>[2x]GSHMSRVQLALRVPDLEASIG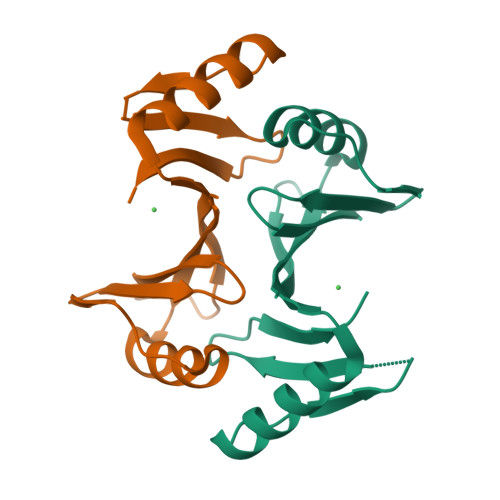FYSKLFGTGPAKVRPGYANFAIAEPPLKLVLIEGAGEDATRLDHLGVEVEDSAQVGHAARRLKESGLATVEENDTACCYAVQDRVWVTGPGGEPWEVYVVKGDAD>[2x]AVFTVVNQCPFTVWAASVPVGGGRQLNRGESWRITAPAGTTAARIWARTGCKFDASGRGSCRTGDCGGVLQCTGYGRAPNTLAEYALKQFNNLDFFDI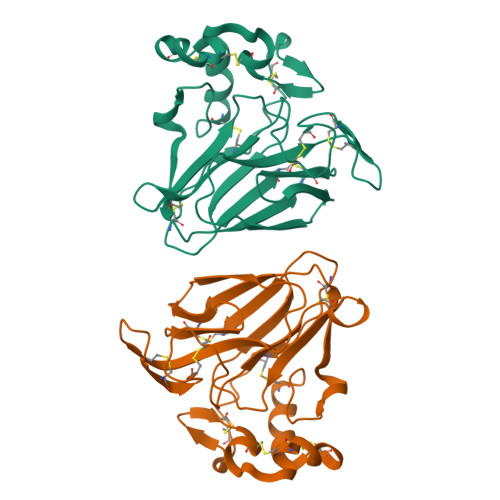SLIDGFNVPMSFLPDGGSGCSRGPRCAVDVNARCPAELRQDGVCNNACPVFKKDEYCCVGSAANDCHPTNYSRYFKGQCPDAYSYPKDDATSTFTCPAGTNYKVVFCP>[2x]MEEPEEPADSGQSLVPVYIYSPEYVSMCDSLAKIPKRASMVHSLIEAYALHKQMRIVKPKVASMEEMATFHTDAYLQHLQKVSQEGDDDHPDSIEYGLGYDCPATEGIFDYAAAIGGATITAAQCLIDGMCKVAINWSGGWHHAKKDEASGFCYLNDAVLGILRLRRKFERILYVDLDLHHGDGVEDAFSFTSKVMTVSLHKFSPGFFPGTGDVSDVGLGKGRYYSVNVPIQDGIQDEKYYQICES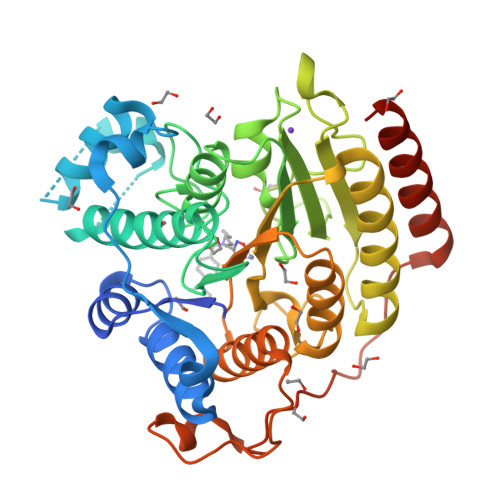VLKEVYQAFNPKAVVLQLGADTIAGDPMCSFNMTPVGIGKCLKYILQWQLATLILGGGAYNLANTARCWTYLTGVILGKTLSSEIPDHEFFTAYGPDYVLEITPSCRPDRNEPHRIQQILNYIKGNLKHVVIEGRGSHHHHHH> GGTIARTIVLQESIGKGRFGEVWRGKWRGEEVAVKIFSSREERSWFREAEIYQTVMLRHENILGFIAADNKDNGTWTQLWLVSDYHEHGSLFDYLNRYTVTVEGMIKLAL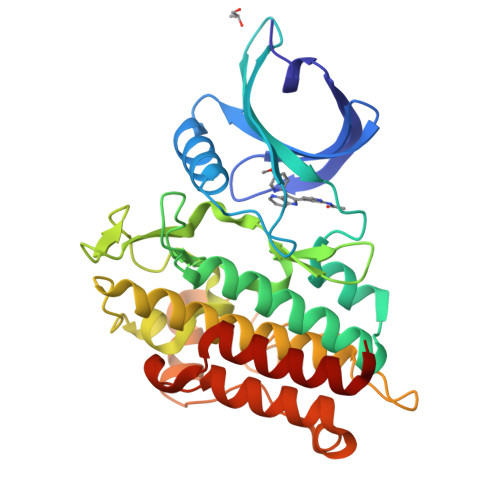STASGLAHLHMEIVGTQGKPAIAHRDLKSKNILVKKNGTCCIADLGLAVRHDSATDTIDIAPNHRVGTKRYMAPEVLDDSINMKHFESFKRADIYAMGLVFWEIARRCSIGGIHEDYQLPYYDLVPSDPSVEEMRKVVCEQKLRPNIPNRWQSCEALRVMAKIMRECWYANGAARLTALRIKKTLSQLSQQEGIKM(2S)-2-oxidanyl-2-[oxidanyl(propan-2-yl)amino]ethanoic acid | C5 H11 N O4 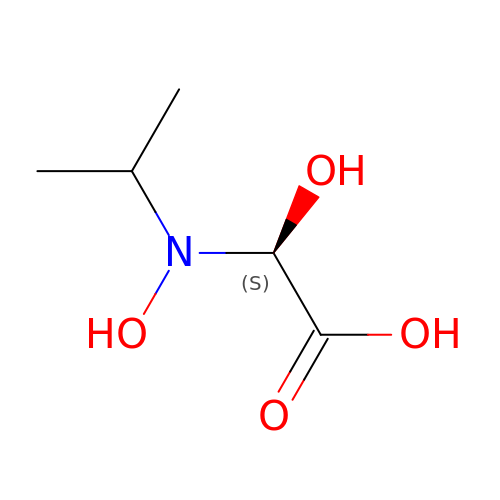| SAXCDYFGYFOTMB-BYPYZUCNSA-N>GAMGSGIHIRKLLLLGAGESGKSTIFKQIKLLFQTGFDEGELKSYVPVIHANVYQTIKLLHDGT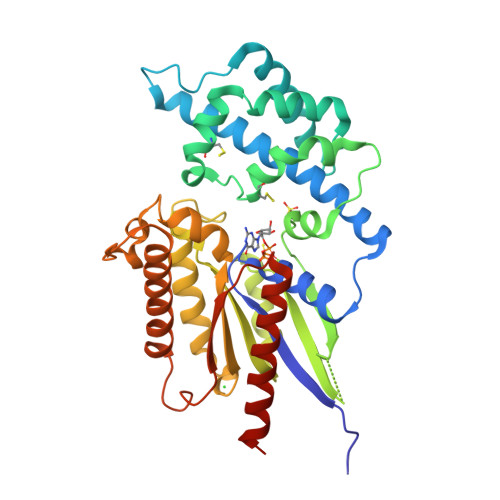KEFAQNETDSAKYMLSSESIAIGEKLSEIGGRLDYPRLTKDIAEGIETLWKDPAIQETCARGNELQVPDCTKYLMENLKRLSDINYIPTKEDVLYARVRTTGVVEIQFSPVGENKKSGEVYRLFDVGGQRNERRKWIHLFEGVTAVIFCAAISEYDQTLFEDEQKNRMMETKELFDWVLKQPCFEKTSFMLFLNKFDIFEKKVLDVPLNVCEWFRDYQPVSSGKQEIEHAYEFVKKKFEELYYQNTAPDRVDRVFKIYRTTALDQKLVKKTFKLVDETLRRRNLLEAGLL[3x]> MTVATTKTREYAEIVYKIAQGFVLSKLSSKH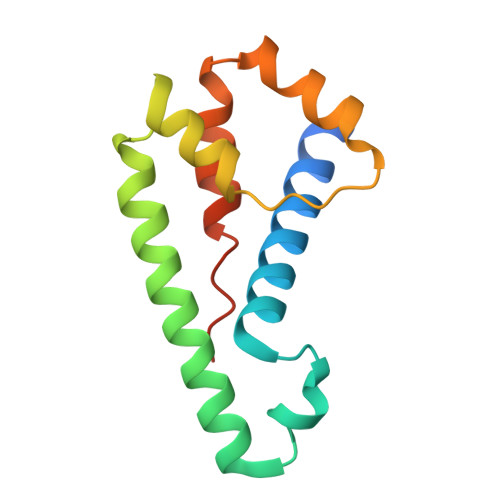DLQWSKCKGNPKLEREYNDKKEKVVNEAFLAIRSRTEKQAFIDYFVSTLYPHVRQDEFVDFAQKLFQDTDEIRSLTLLALSSQYPIKRQGETE The human (Homo sapiens; Hs) methyltransferase (MTase) METTL9 is the first enzyme shown to generate 1-methylhistidine (π-methylhistidine) in proteins. METTL9 preferentially methylates an alternating histidine (HxH) motif, where “x” is a small, uncharged amino acid, and multiple substrates have been identified. METTL9 belongs to the so-called seven β-strand (7BS) MTase family, also referred to as Class I or Rossmann-like MTases. Putative METTL9 orthologues are found in most eukaryotes, and we have here investigated the activity of such enzymes from several species, representing all five eukaryotic supergroups.

To investigate whether any structural differences could explain the distinct substrate specificity of OtMETTL9, we solved its apo crystal structure and compared it to the recently published structures of HsMETTL9 (16, 17). Like HsMETTL9, the OtMETTL9 structure is a monomer, adopting the canonical 7BS MTase fold consisting of seven β-strands (β1-β7) that form a twisted sheet of characteristic topology, alternating with six α helices (α1-α6) located on both sides of the β-sheet. The overall structure is very similar to HsMETTL9 with a root-mean square deviation (RMSD) of only 2.1 Å. Like HsMETTL9, OtMETTL9 contains additional structural elements (β′1-β′3, α′1-α′4) outside of the core 7BS fold, which are typically involved in substrate recognition. Among them, the region containing β′2-β′3 has a slightly different orientation in OtMETTL9 than in HsMETTL9 as will be discussed later. We also noticed that the binding surface of OtMETTL9 could instead extend into an adjacent side pocket, where peptide residues located C-terminally of the HxH-motif could bind, creating a bent, C-shaped, binding groove, as opposed to the straight groove of HsMETTL9. For HsMETTL9, access to this side pocket is blocked by strands β′2 and β′3, which are positioned differently from OtMETTL9. Binding of the peptide in the C-shaped groove in OtMETTL9 may impose additional constraints on the identity of the Xc residue, which may explain the more stringent requirement (small residues G or S) for peptide methylation activity of the OtMETTL9 enzyme as compared to HsMETTL9. Most of the residues that are in contact with the X or XN positions in the HsMETTL9 structures are identical and have a similar orientation in the OtMETTL9 structure, such as N88 (Hs N118), R93 (Hs R123), G94 (Hs G124), M96 (Hs M126), R198 (Hs R214), D286 (Hs D300), and Y292 (Hs Y306), whereas S283 has similar properties to the human C297. The only difference is OtMETTL9 L84, corresponding to the human R114, which moves upon peptide binding and interacts with both X and XN.

> GPLGSMASEERTSALRIRCAHCDAVFDERALPYDADVDSLASSALREKFVRLSLDSESVEFLNRARARGRDECERLARKCTELRRTMSLTEANAILGRGKMFVFSDAHVETLMRACGEGAGGGWFLDVGAGEGEVTRTLARRFAGTCATESSPGMASRLREKGFDVVLESDTVENVVRETRARGGDVSEDGFDVVAALNLCDRVRSPRALLRDLKRALKAKTGILILAIVVPFRPFVENADGTRSQPDERLDVPSAGSWESGVDALWTELIAPLGFDLVTLSRVPYISEGDHLYDAYVLDDAVFVLRAPP>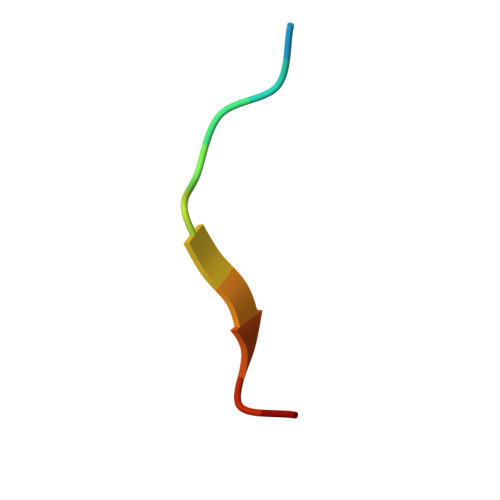 QEEEGSAGGQGG> MATDMQRKRSSECLDGTLTPSDGQSMERAESPTPGMAQGMEPGAGQEGAMFVHARSYEDLTESEDGAASGDSHKEGTRGPPPLPTDMRQISQDFSELSTQLTGVARDLQEEMLPGSSEDWLEPPGAVGRPATEPPREGTTEGDEEDATEAWRLHQKHVFVLSEAGKPVYSRYGSEEALSSTMGVMVALVSFLEADKNAIRSIHADGYKVVFVRRSPLVLVAVARTRQSAQELAQELLYIYYQILSLLTGAQLSHIFQQKQNYDLRRLLSGSERITDNLLQLMARDPSFLMGAARCLPLAAAVRDTVSASLQQARARSLVFSILLARNQLVALVRRKDQFLHPIDLHLLFNLISSSSSFREGEAWTPVCLPKFNAAGFFHAHISYLEPDTDL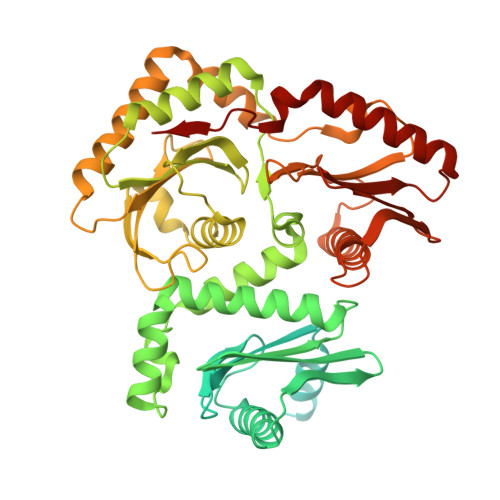CLLLVSTDREDFFAVSDCRRRFQERLRKRGAHLALREALRTPYYSVAQVGIPDLRHFLYKSKSSGLFTSPEIEAPYTSEEEQERLLGLYQYLHSRAHNASRPLKTIYYTGPNENLLAWVTGAFELYMCYSPLGTKASAVSAIHKLMRWIRKEEDRLFILTPLTY5-{(2E,4aR,7aR)-6-[5-fluoro-4-methyl-6-(methylamino)pyrimidin-2-yl]-2-imino-3-methyl-4-oxooctahydro-7aH-pyrrolo[3,4-d]pyrimidin-7a-yl}thiophene-2-carbonitrile 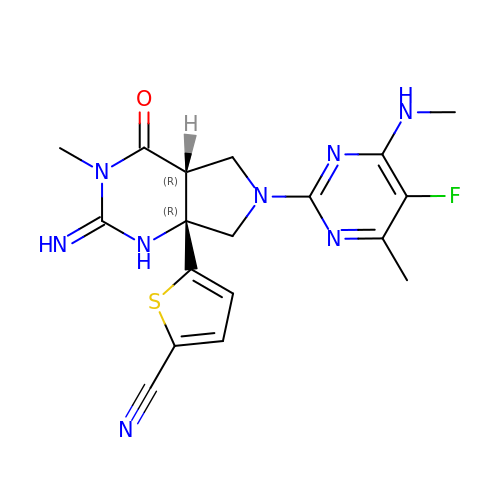| C18 H19 F N8 O S | ZGUINBOSNMEMBB-VOJFVSQTSA-N3-chlorobenzene-1,2-diol | C6 H5 Cl O2 | 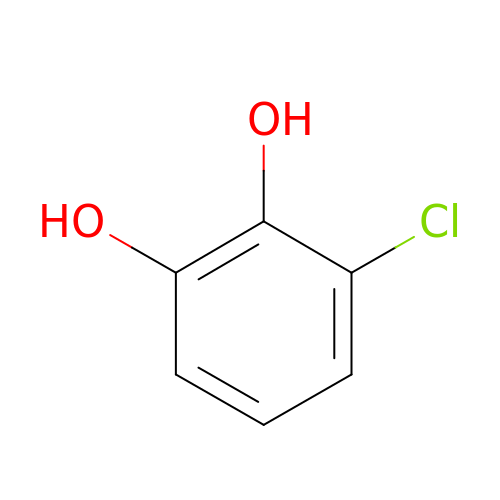GQKDZDYQXPOXEM-UHFFFAOYSA-N2-[[3-[(3-aminophenyl)carbamoyl]phenyl]amino]-~{N}-(2-chloranyl-6-methyl-phenyl)-1,3-thiazole-5-carboxamide | C24 H20 Cl N5 O2 S | 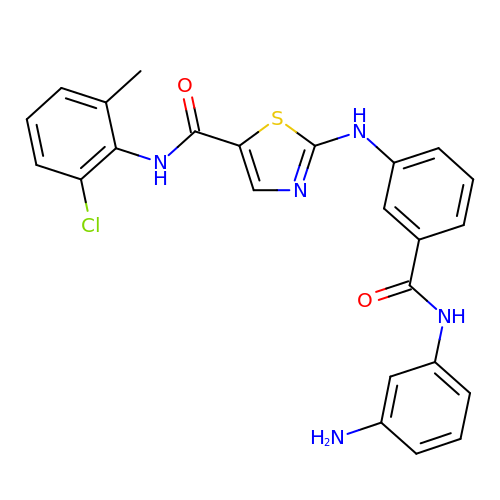LNMMQCKJDHNCQP-UHFFFAOYSA-N> MPKRTDIKSILILGAGPIVIGQACEFDYSGAQACKALREEGYRVILVNSNPATIMTDPEMADATYIEPIHWEVVRKIIEKERPDAVLPTMGGQTALNCALELERQGVLEEFGVTMIGATADAIDKAEDRRRFDVAMKKIGLETARSGIAHTMEEALAVAADVGFPCIIRPSFTMG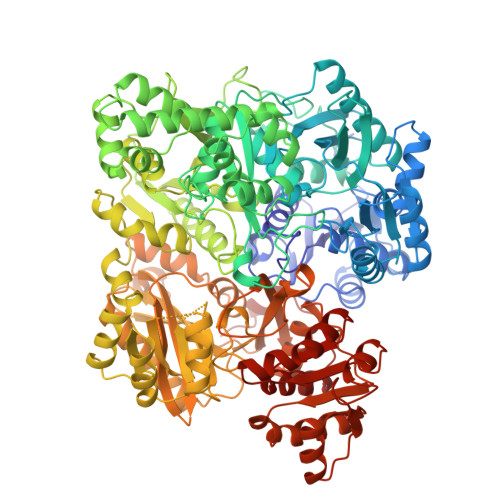GSGGGIAYNREEFEEICARGLDLSPTKELLIDESLIGWKEYEMEVVRDKNDNCIIVCSIENFDAMGIHTGDSITVAPAQTLTDKEYQIMRNASMAVLREIGVETGGSNVQFAVNPKNGRLIVIEMNPRVSRSSALASKATGFPIAKVAAKLAVGYTLDELMNDITGGRTPASFEPSIDYVVTKIPRFNFEKFAGANDRLTTQMKSVGEVMAIGRTQQESLQKALRGLEVGATGFDPKVSLDDPEALTKIRRELKDAGADRIWYIADAFRAGLSVDGVFNLTNIDRWFLVQIEELVRLEEKVAEVGITGLNADFLRQLKRKGFADARLAKLAGVREAEIRKLRDQYDLHPVYKRVDTCAAEFATDTAYMYSTYEEECEANPSTDREKIMVLGGGPNRIGQGIEFDYCCVHASLALREDGYETIMVNCNPETVSTDYDTSDRLYFEPVTLEDVLEIVRIEKPKGVIVQYGGQTPLKLARALEAAGVPVIGTSPDAIDRAEDRERFQHAVERLKLKQPANATVTAIEMAVEKAKEIGYPLVVRPSYVLGGRAMEIVYDEADLRRYFQTAVSVSNDAPVLLDHFLDDAVEVDVDAICDGEMVLIGGIMEHIEQAGVHSGDSACSLPAYTLSQEIQDVMRQQVQKLAFELQVRGLMNVQFAVKNNEVYLIEVNPRAARTVPFVSKATGVPLAKVAARVMAGKSLAEQGVTKEVIPPYYSVKEVVLPFNKFPGVDPLLGPEMRSTGEVMGVGRTFAEAFAKAQLGSNSTMKKHGRALLSVREGDKERVVDLAAKLLKQGFELDATHGTAIVLGEAGINPRLVNKVHEGRPHIQDRIKNGEYTYIINTTSGRRAIEDSRVIRRSALQYKVHYDTTLNGGFATAMALNADATEKVISVQEMHAQIK There have been increased efforts recently to “drug” RNA using orally bioavailable, low-molecular-weight compounds. This study combines two of the most powerful tools of modern drug discovery, high-throughput screening and structure-based design, to target the theophylline aptamer, a tertiary-structured RNA that binds theophylline with high affinity and selectivity. That structure revealed how multiple interdependent components of the RNA form a well-defined ligand binding pocket that enables theophylline to bind with submicromolar affinity while excluding closely related compounds such as caffeine (which differs by a single methyl group) by more than 10,000-fold. Previous biophysical and modeling studies have shown that the aptamer undergoes a large conformational rearrangement upon binding theophylline. X-ray crystal structures were determined for the aptamer, both in isolation and in complex with various ligands, revealing the molecular basis for ligand binding.

One of the hit compounds, theophylline aptamer ligand 1 (TAL1), is an aminomethyl-substituted pteridinone that has a similar molecular weight as that of theophylline. The tightest binder is TAL1, with a Kd that is 340-fold lower than that of theophylline. The second strategy involved replacing the G2–U32 wobble pair at the base of the RNA aptamer by a G–C Watson–Crick pair, thus stabilizing the corresponding stem. Thus, to reveal atomic-level details of the RNA–ligand interaction, it was necessary to turn to the second crystallization strategy, with the stabilized aptamer stem and no protein component. This approach gave high-quality crystals (1.42–2.70 Å resolution) for the various aptamer–ligand complexes. The highest-affinity ligand that emerged from the screen is TAL1, which gave crystals that contain four complexes in the asymmetric unit, providing excellent electron density information for the bound ligand. This compound binds in a similar manner to theophylline and TAL2 but forms two additional hydrogen bonds with the RNA. C22 is again engaged through N3 and the exocyclic amine, as well as a third interaction with O2. U24 is again engaged through N3, as well as a second interaction with O2. In order to accommodate TAL1 within the pocket, U24 is rotated outward by 0.7 Å compared to its orientation in the theophylline-bound complex. TAL1 and the dimethoxy-quinazolinone core of the other three hits have a molecular weight of 193.1 and 206.2 Da, respectively, which is similar to that of theophylline (180.2 Da), thus demonstrating good ligand efficiency to achieve a Kd as low as 2.0 nM for binding to the RNA.

>GGCGAUACCAGCCGAAAGGCCCUUGGCAGCGCC[4x]>EAEAAGLNTAAKAKGLKYFGSATDNPELTDSAYVAQLSNTDDFGQITPGNSMKWDATEPSQNSFSFANGDAVVNLANKNGQLMRCHTLVWHSQLPNWVSSGSWTNATLLAAMKNHITNVVTHYKGKCYAWDVVNEALNEDGTFRNSVFYQIIGPAYIPIAFATAAAADPDVKLYYNDYNIEYSGAKATAAQNIVKMIKAYGAKIDGVGLQAHFIVGSTPSQSDLTTVLKGYTALGVEVAYTELDIKMQLPSTAAKL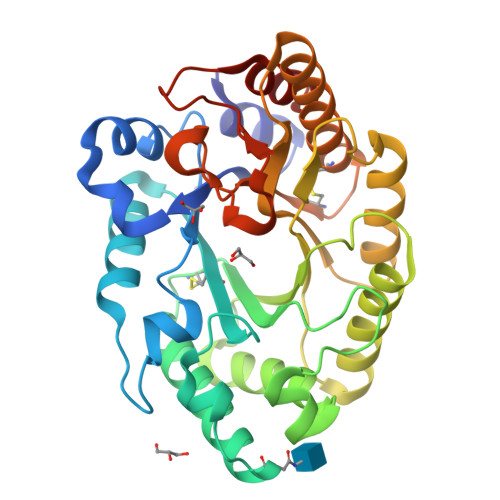AQQSTDFQGVAAACVSTTGCVGVTIWDWTDKYSWVPSVFQGYGAPLPWDENYVKKPAYDGLMAGLGASGSGTT[2x]> VLQLKLGNSAIVTQEAANMCCAYGEWPSYLPDNEATAIDKPTQPETSTDRFYTLKSVK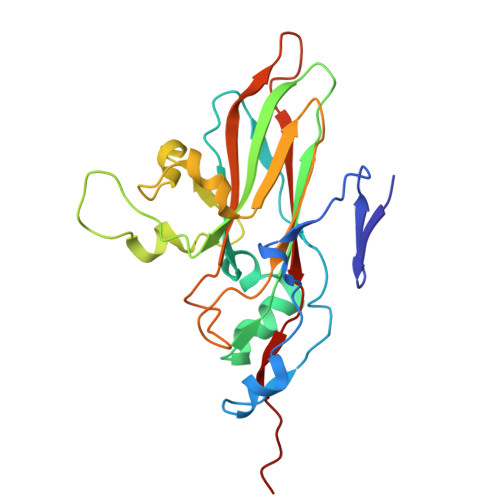WEGTSTGWWWKLPDALNQTGMFGQNVQYHYLYRSGFLCHVQCNATKFHQGALLVVAIPEHQLGKYNTGTSASFDDVMKGKTGGVFTHPYVLDDGTSLACSLIFPHQWINLRTNNSATIMLPWMNCAPMDFALRHNQWTLAIIPVVPLNTSGGTTMVPITVSIAPMCCEFNGLRNAIT> MTTTMKISIEFLEPFRMTKWQESTRRNKNNKEFVRGQAFARWHRNKKDNTKGRPYITGTLLRSAVIRSAENLLTLSDGKISEKTCCPGKFDTEDKDRLLQLRQRSTLRWTDKNPCPDNAETYCPFCELLGRSGNDGKKAEKKDWRFRIHFGNLSLPGKPDFDGPKAIGSQRVLNRVDFKSGKAHDFFKAYEVDHTRFPRFEGEITIDNKVSAEARKLLCDSLKFTDRLCGALCVIRFDEYTPAADSGKQTENVQAEPNANLAEKTAEQIISILDDNKKTEYTRLLADAIRSLRRSSKLVAGLPKDHDGKDDHYLWDIGKKKKDENSVTIRQILTTSADTKELKNAGKWREFCEKLGEALYLKSKDMSGGLKITRRILGDAEFHGKPDRLEKSRSVSIGSVLKETVVCGELVAKTPFFFGAIDEDAKQTALQVLLTPDNKYRLPRSAVRGILRRDLQTYFDSPCNAELGGRPCMCKTCRIM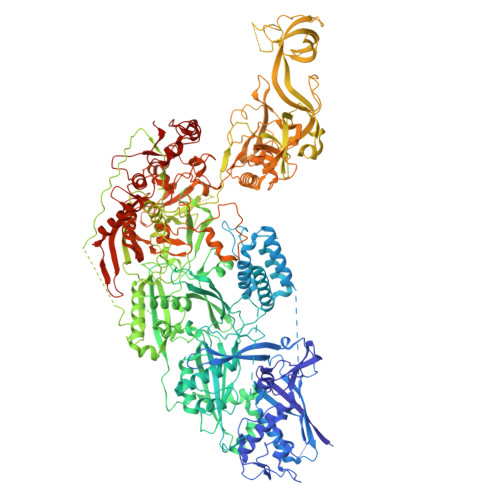RGITVMDARSEYNAPPEIRHRTRINPFTGTVAEGALFNMEVAPEGIVFPFQLRYRGSEDGLPDALKTVLKWWAEGQAFMSGAASTGKGRFRMENAKYETLDLSDENQRNDYLKNWGWRDEKGLEELKKRLNSGLPEPGNYRDPKWHEINVSIEMASPFINGDPIRAAVDKRGTAVVTFVKYKAEGEEAKPVCAYKAESFRGVIRSAVARIHMEDGVPLTELTHSDCECLLCQIFGSEYEAGKIRFEDLVFESDPEPVTFDHVAIDRFTGGAADKKKFDDSPLPGSPARPLMLKGSFWIRRDVLEDEEYCKALGKALADVNNGLYPLGGKSAIGYGQVKSLGIKGDDKRISRLMNPAFDETDVAVPEKPKTDAEVRIEAEKVYYPHYFVEPHKKVEREEKPCGHQKFHEGRLTGKIRCKLITKTPLIVPDTSNDDFFRPADKEARKEKDEYHKSYAFFRLHKQIMIPGSELRGMVSSVYETVTNSCFRIFDETKRLSWRMDADHQNVLQDFLPGRVTADGKHIQKFSETARVPFYDKTQKHFDILDEQEIAGEKPVRMWVKRFIKRLSLVDPAKHPQKKQDNKWKRRKEGIATFIEQKNGSYYFNVVTNNGCTSFHLWHKPDNFDQEKLEGIQNGEKLDCWVRDSRYQKAFQEIPENDPDGWECKEGYLHVVGPSKVEFSDKKGDVINNFQGTLPSVPNDWKTIRTNDFKNRKRKNEPVFCCEDDKGNYYTMAKYCETFFFDLKENEEYEIPEKARIKYKELLRVYNNNPQAVPESVFQSRVARENVEKLKSGDLVYFKHNEKYVEDIVPVRISRTVDDRMIGKRMSADLRPCHGDWVEDGDLSALNAYPEKRLLLRHPKGLCPACRLFGTGSYKGRVRFGFASLENDPEWLIPGKNPGDPFHGGPVMLSLLERPRPTWSIPGSDNKFKVPGRKFYVHHHAWKTIKDGNHPTTGKAIEQSPNNRTVEALAGGNSFSFEIAFENLKEWELGLLIHSLQLEKGLAHKLGMAKSMGFGSVEIDVESVRLRKDWKQWRNGNSEIPNWLGKGFAKLKEWFRDELDFIENLKKLLWFPEGDQAPRVCYPMLRKKDDPNGNSGYEELKDGEFKKEDRQKKLTTPWTPWASSGLVPRGSHHHHHHH>[6x]MRLSYEALEWRTPIENSTEPVSLPPPPPFFGQERAREALELAIRGGFHAYLVGPPSLGKHEALLAYLSTQSVETPPDLLYVPLSERKVAVLTLPSGQEIHLAEAVEGLLLEVNRLDELFRQGSFLREKTQLEARFKEAREQQLEALRREAQEAGFALSTNGERLELTGPGPVPAELSARLEEVTLGSLAASAELEVALRRLRRDWALHYLNNRFEPLFQRFPQARAYLEALRARLARYAETGEPLDPAQWRPNLLTSSSSGTPPPIVYEPYATAPRLFGRLDYLVDRGVWSTNVSLIRPGAVHRAQGGYLILDALSLKREGTWEAFKRALRNGQVEPVTEPQAPAGLEVEPFPIQMQVILVGTPEAFEGLEEDPAFSELFRIRAE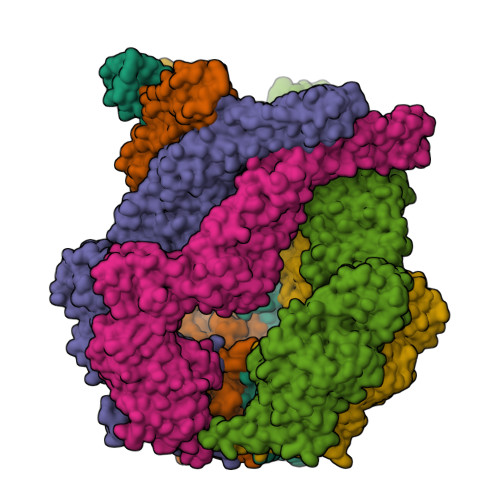FSPTLPASPENCTALGGWLLAQGFQLTQGGLTRLYDEARRMAEQRDRMDARLVEIRALAEEAAVLGGGLLTAESVEQAIAAREHRSFLSEEEFLRAVQEGVIRLRTTGRAVGEVNSLVVVEAAPYWGRPARLTARAAPGRDHLISIDREAGLGGQIFHKAVLTLAGYLRSRYIEHGSLPVTISLAFEQNYVSIEGDSAGLAELVAALSAIGNLPLRQDLAVTGAVDQTGKVLAVGAINAKVEGFFRVCKALGLSGTQGVILPEANLANLTLRAEVLEAVRAGQFHIYAVETAEQALEILAGARMEGFRGLQEKIRAGLEAFARLEEGHDKEDREKLAAALEHHHHHH>GSVIDVSSQRVNVQRPLD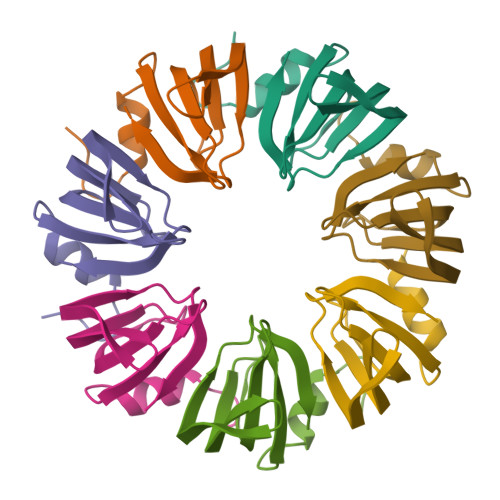ALGNSLNSPVIIKLKGDREFRGVLKSFDLHMNLVLNDAEELEDGEVTRRLGTVLIRGDNIVYISP[7x]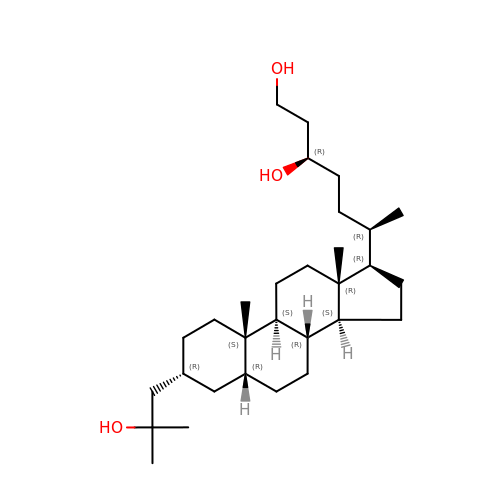(3R,6R)-6-[(3R,5R,8R,9S,10S,13R,14S,17R)-10,13-dimethyl-3-(2-methyl-2-oxidanyl-propyl)-2,3,4,5,6,7,8,9,11,12,14,15,16,17-tetradecahydro-1H-cyclopenta[a]phenanthren-17-yl]heptane-1,3-diol | C30 H54 O3 | BELGEHMGZKEZEK-JSCSUZHRSA-N1-[2-chloranyl-7-[(1~{R},2~{R})-1,2-dimethoxypropyl]pyrazolo[1,5-a]pyrimidin-6-yl]-3-[5-chloranyl-6-(1,2,3-triazol-2-yl)pyridin-3-yl]urea 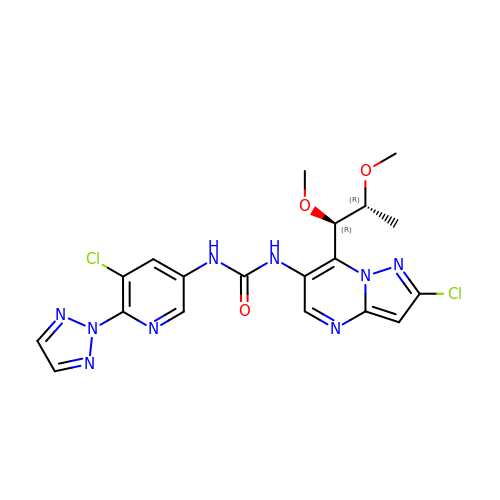| C19 H19 Cl2 N9 O3 | XKQLNDPUQSZBJW-QGHHPUGFSA-N>[2x]MHHHHHHTLGDQGGQGQEPPPEPRITLKVGGQPVTFLVDTGAQHSVLTQNPGPLSDKSAWVQGATGGKRYRWTTDRKVHLATGKVTHSFLHVPDCPYP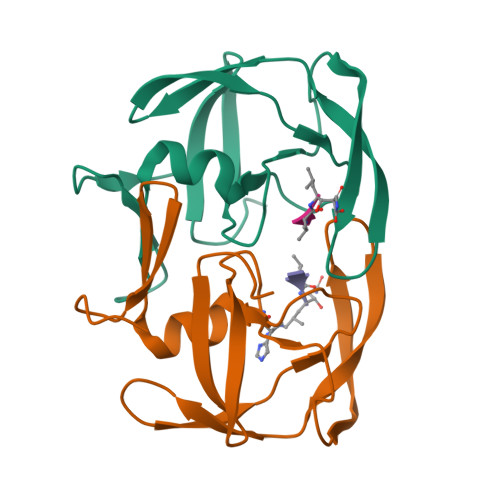LLGRDLLTKLKAQIHFEGSGAQVVGPMGQPLQVL>[2x]MSLGVTMHDVAKAAGVSAITVSRVLNQPQQVSEQLREKVMQAVDALAYVPSRSASTLASAKSRTVLVLIP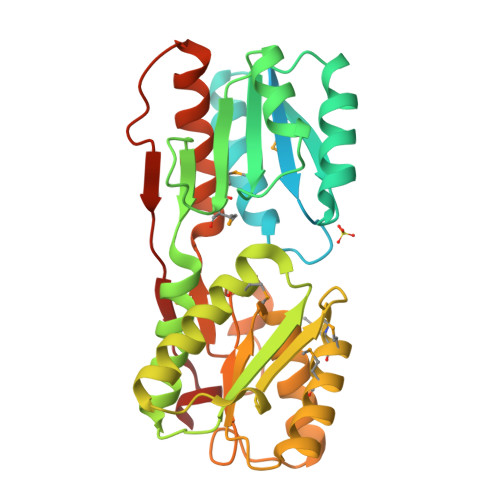SLANTVFLETLTGIETVLDAAGYQMLIGNSHYDAGQELQLLRAYLQHRPDGVLITGLSHAEPFERILSQHALPVVYMMDLADDGRCCVGFSQEDAGAAITRHLLSRGKRRIGFLGAQLDERVMKRLDGYRAALDAADCRDAGLEWLDPQPSSMQMGADMLDRALAERPDCDALFCCNDDLAIGALARSQQLGIAVPERLAIAGFNDLQPAAWCTPPLTTVATPRRDIGVHAAKALLQLIDGEEPASRRADLGFRLMLRRSSEGHHHHHH> MAYEAQYYPGATSVGANRRKHMSGKLEKLREISDEDLTAVLGHRAPGSDYPSTHPPLAEMGEPACSIREAVAATPGAAAGDRVRYVQFADSMYNAPATPYFRSYFAAINFRGVDPGTLSGRQIVEARERDMEQCAKVQMETEMTDPALAGMRGATVHGHSVRLQEDGVMFDMLDRRRLEGGVIIMDKDQVAIPLDRKVNLGKPMSSEEAAKRTTIYRVDNVAFRDDAEV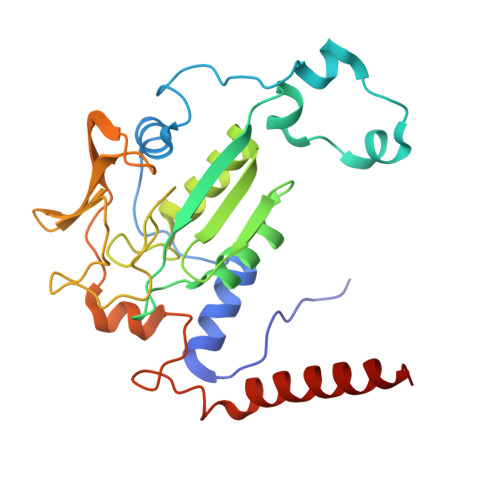IEWVHRVFDQRTSYGFQPK> MASSRSELLLDRFAEKIGVGSISFNENRLCSFAIDEIYYISLSDANDEYMMIYGVCGKFPTDN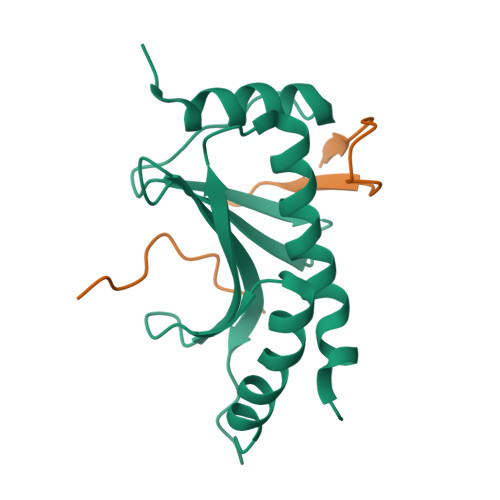PNFALEILNANLWFAENGGPYLCYESGAQSLLLALRFPLDDATPEKLENEIEVVVKSMENLYLVLHNQGITLENEH;> MGSSHHHHHHSQDPGGTGHLISSTGALGSRSLFSPLRNSMADSVDSRDIPGLPTNPSRLAAAT> GTTNTVAAYNLTWKSTNFKTILEWEPKPVNQVYTVQISTKSGDWKSKCFYTTDTECDLTDEIVKDVKQTYLARVFSYPAGNVESTGSAGEPLYENSPEFTPYLETNLGQPTIQSFEQVGTKVNVTVEDERTLVRRNNTFLSLRDVFGKDL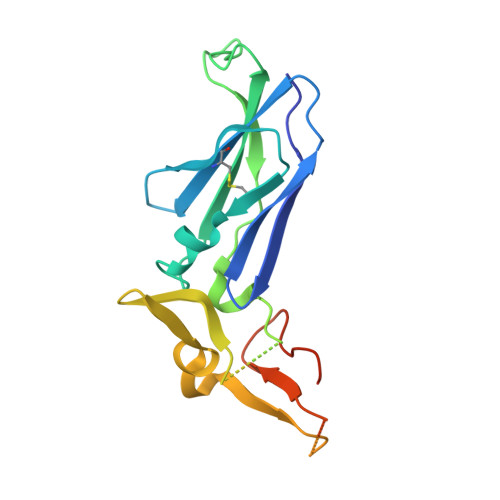IYTLYYWKSSSSGKKTAKTNTNEFLIDVDKGENYCFSVQAVIPSRTVNRKSTDSPVECMGQEKGEFRE>[2x]CCG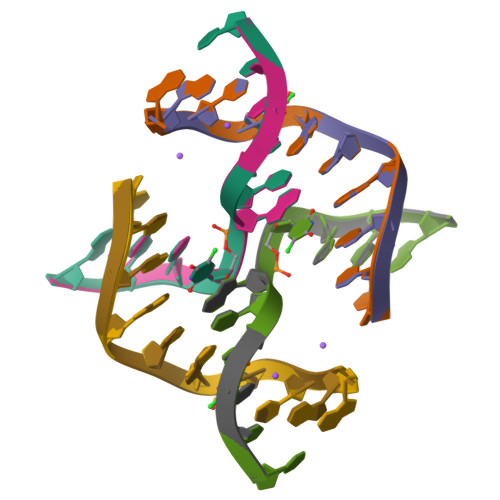GTAUCGG;>CCGATACCGG[2x]> MFRRTFFTPMIAQPTLLMLGNKGGTPKRKKNPMQL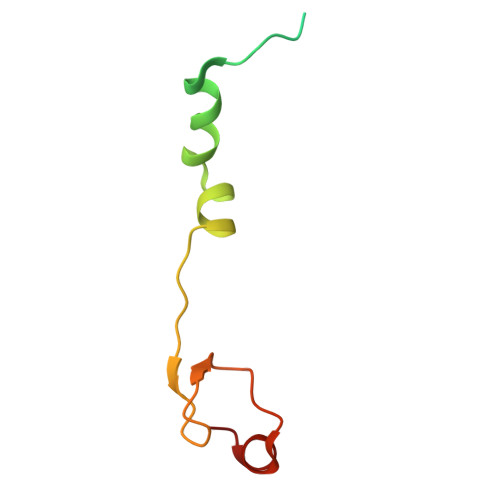RRKVYGLHFKEKYLKMEEWYYCPLCAEPKKPGEWCRREDCRQIKP3-(2,4-diamino-6-methylquinazolin-7-yl)-4-ethoxybenzaldehyde | C18 H18 N4 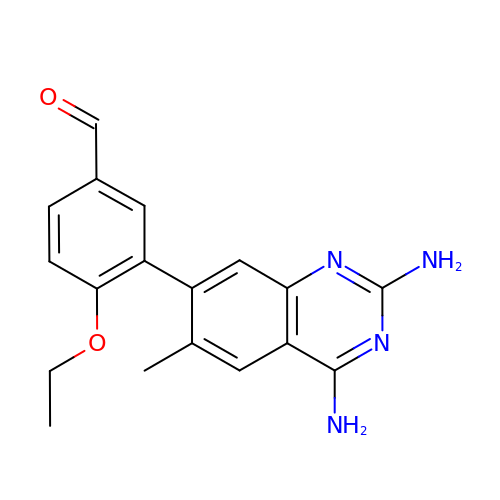O2 | BDVALXKNVWZHIQ-UHFFFAOYSA-N Proliferating Cell Nuclear Antigen (PCNA)—the eukaryotic sliding clamp—is an 86-kDa homotrimeric ring with a six-fold pseudosymmetric rotation axis running through the centre of the clamp and a central channel lined with lysine and arginine-rich α-helices through which DNA is threaded (1–6). The front face of the PCNA ring contains the site of interaction of polymerases and other proteins, named the PIP-box binding site. The PCNA–associated factor p15PAF (hereafter named p15) is an oncogenic, 11 kDa intrinsically disordered protein that regulates DNA replication and lesion bypass via a PIP-box interaction with PCNA. p15 co-localizes with PCNA in the nucleus of proliferating cells mainly in the S phase of the cell cycle. Thus, p15 outcompetes DNA for a common binding site in the clamp channel, and the stoichiometry of binding dictates the available sliding surfaces.

In the electron density map, however, no significant density was observed that may arise from DNA, suggesting that, although incorporated in the crystal, the DNA is not sufficiently ordered to generate a structured signal. The electron density map showed three p15 fragments spanning residues 50–72 in the corresponding PIP-box sites, with a conformation analogous to that observed in the co-structure with the p1550–77 peptide. Notably, due to steric hindrance, the location of the p1541–72 peptides would interfere with DNA binding to PCNA in the orientation observed in the PCNA–dsDNA binary structure, suggesting that p15 may outcompete DNA for binding to the PCNA inner rim. Accordingly, when PCNA is co-crystallized with three p15 peptides and DNA, the electron density map does not show features of DNA in the clamp channel. Critically, p15 shields key residues at the PCNA sliding surfaces, confining DNA in discrete positions, which depend on the p15 stoichiometry of binding. This mode of binding, with DNA partially competing with p15 for a single binding site on the clamp inner ring, is also supported by (i) our NMR study showing that DNA does not disengage p15 from the inner wall of PCNA saturated with p15 and (ii) our structure of PCNA co-crystallized with three p15 peptides and DNA, showing that DNA does not occupy the central channel.

>GPHMFEARLVQGSILKKVLEALKDLINEACWDISSSGVNLQSMDSSHVSLVQLTLRSEGFDTYRCDRNLAMGVNLTSMSKILKCAGNEDIITLRAEDNADTLALVFEAPNQEKVSDYEMKLMDLDVEQLGIPEQEYSCVVKMPSGEFARICRDLSHIGDAVVISCAKDGVKFSASGELGNGNIKLSQTSNVDKEEEAVTIEMNEPVQLTFALRYLNFFTKATPLSSTVTLSMSADVPLVVEYKIADMGHLKYYLAPKIEDEEGS[3x];>RKAENKYAGGNPVCVRPTPKWQKGIGEFFRLS[3x]>GAMAKVQVNNVVVLDNPSPFYNPFQFEITFECIEDLSEDLEWKIIYVGSAESEEYDQVLDSVLVGPVPAGRHMFVFQADAPNPGLIPDADAVGVTVVLITCTYRGQEFIRVGYYVNNEYTETELRENPPV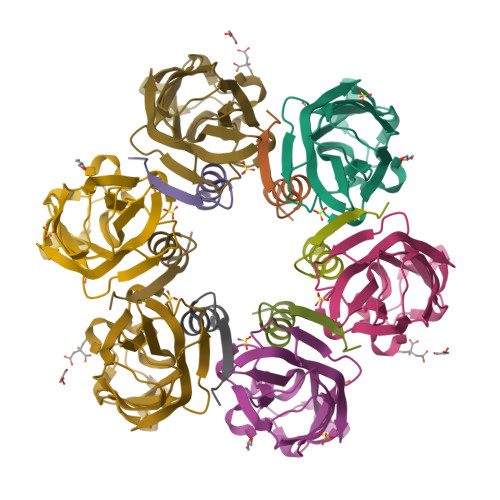KPDFSKLQRNILASNPRVTRFHINWEDN[2x];>ASTEEKWARLARRIAGAGGVTLDGFG[2x]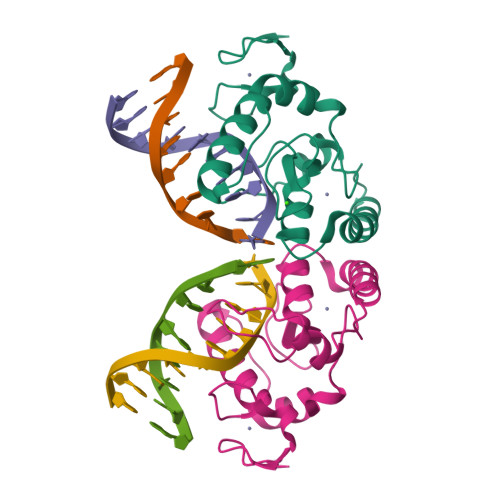> MTQCPRCQRNLAADEFYAGSSKMCKGCMTWQNLSYNANKEGHANTFTKATFLAWYGLSAQRHCGYCGISEAGFTSLHRTNPRGYHIQCLGVDRSDSFEGYSPQNARLACFICNRIKSNIFSASEMDVLGEAISKAWHGRGIA> SWQTYVDEHLMCDIDGQGQQLAASAIVGHDGSVWAQSSSFPQFKPQEITGIMKDFEEPGHLAPTGLHLGGIKYMVIQGEAGAVIRGKKGSGGITIKKTGQALVFGIYEEPVTPGQCNMVVERLGDYLIDQGL

Bet v 2 is a plant profilin panallergen, i.e., it is ubiquitously distributed throughout nature and shares a highly conserved amino acid sequence of up to 75% even between distantly-related organisms. Additionally to its ability to bind actin, profilins also interact with poly-l-proline and phosphoinositides. In this study, we present crystal structures of Bet v 2 in the reduced (without disulfide bridge) and the oxidized (with disulfide bridge) states at a resolution of 2.0 and 1.7 Å respectively. The reduced and oxidized structures were determined at a high resolution of 2.0 Å and 1.7 Å, respectively. Both structures share a central six-stranded antiparallel β-sheet with two N- and the C-terminal α-helices flanking the sheet at one side and a third helix flanking the sheet on the opposite side.

While the overall structure was conserved between these two forms, the crystal structures revealed marked differences near the N- and C-terminal segments, which are linked by the disulfide bridge Cys13-Cys117. In the oxidized form, the N-terminal segment is disulfide linked to the C-terminal helix, which adopts a strained conformation enforced by the disulfide bond. The poly-l-proline binding sites of Bet v 2 map onto the immediate neighborhood of the Cys13-Cys117 disulfide bond, providing a direct link between the differences in proline binding with the differences in the crystal structures of both Bet v 2 forms. Hence, the apparent higher binding ability to poly-l-proline of the oxidized Bet v 2 can be explained by the conformational selection principle: the likelihood for the ligand to find the receptor in a conformation suitable for binding is increased if the conformational space of the receptor is restricted by a disulfide bridge. In this work, we showed that cathepsin S degrades the reduced form of Bet v 2 rapidly, whereas the processing of the oxidized form is sufficiently retarded. Given the significantly higher proteolytic resistance of oxidized Bet v 2, we suggest that this form is the sensitizing allergen. Importantly, however, the two redox forms differed strongly with respect to their proteolytic resistance, which can have major impacts on the immunologic properties of Bet v 2 for several reasons: firstly, given the long storage times of birch pollen proteins before the contact with a patient, the preferential degradation of the reduced Bet v 2 will accumulate the oxidized Bet v 2 form, resulting in a preferential exposure of patients with the more stable oxidized Bet v 2 form.>[2x]VTSEAYVSGMLFCLGIFLSFYLLTVLLACWENWRQKKKTLLVAIDRA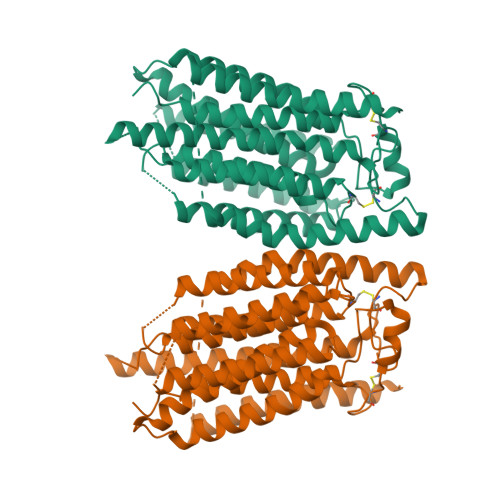CPESGHPRVLADSFPGSSPYEGYNYGSFENVDTLTDIDSDKNVIRTKQYLYVADLARKDKRVLRKKYQIYFWNIATIAVFYALPVVQLVITYQTVVNVTGNQDICYYNFLCAHPLGNLSAFNNILSNLGYILLGLLFLLIILQREINHNRALLRNDLCALECGIPKHFGLFYAMGTALMMEGLLSACYHVCPNYTNFQFDTSFMYMIAGLCMLKLYQKRHPDINASAYSAYACLAIVIFFSVLGVVFGKGNTAFWIVFSIIHIIATLLLSTQLYYMGRWKLDSGIFRRILHVLYTDCIRQCSGPLYVDRMVLLVMGNVINWSLAAYGLIMRPNDFASYLLAIGICNLLLYFAFYIIMKLRSGERIKLIPLLCIVCTSVVWGFALFFFFQGLSTWQKTPAESREHNRDCILLDFFDDHDIWHFLSSIAMFGSFLVLLTLDDDLDTVQRDKIYVFDYKDHDGDYKDHDIDYKDDDDK>[3x]MERPQLDSMSQDLSEALKEATKEVHIRAENSEFMRNFQKGQVSREGFKLVMASLYHIYTALEEEIERNKQNPVYAPLYFPEELHRRAA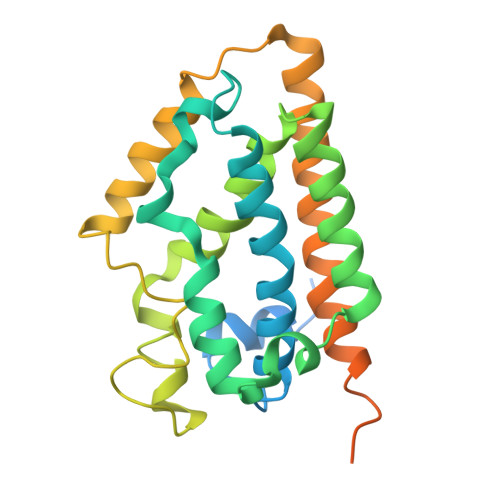LEQDMAFWYGPHWQEAIPYTPATQHYVKRLHEVGGTHPELLVAHAYTRYLGDLSGGQVLKKIAQKAMALPSSGEGLAFFTFPSIDNPTKFKQLYRARMNTLEMTPEVKHRVTEEAKTAFLLNIELFEELQALLTEEHKDQSPSQTEFLRQRPASLVQDTTSAETPRGKSQISTSSSQTP> GGDPHMMFGKKKNNGGSSTARYSAGNKYNTLSNNYALSAQQLLNASKIDDIDSMMGFERYVPPQYNGRFDAKDIDQIPGRVGWLTNMHATLVSQETLSSGSNGGGNSNDGERVTTNQGISGVDFYFLDEEGGSFKSTVVYDPYFFIACNDESRVNDVEELVKKYLESCLKSLQIIRKEDLTMDNHLLGLQKTLIKLSFVNSNQLFEARKLLRPILQDNANNNVQRNIYNVAANGSEKVDAKHLIEDIREYDVPYHVRVSIDKDIRVGKWYKVTQQGFIEDTRKIAFADPVVMAFDIETTKPPLKFRDSAVDQIMMISYMIDGEGFLITNREIISEDIEDFEYTPKPEYPGFFTIFNENDEVALLQRFFEHIRDVRPTVISTFNGDFFDWPFIHNRSKIHGLDMFDEIGFAPDAEGEYKSSYCSHMDCFRWVKRDSYLPQGSQGLKAVTQSKLGYNPIELDPELMTPYAFEKPQHLSEYSVSDAVATYYLYMKYVHPFIFSLCTIIPLNPDETLRKGTGTLCEMLLMVQAYQHNILLPNKHTDPIERFYDGHLLESETYVGGHVESLEAGVFRSDLKNEFKIDPSAIDELLQELPEALKFSVEVENKSSVDKVTNFEEIKNQITQKLLELKENNIRNELPLIYHVDVASMYPNIMTTNRLQPDSIKAERDCASCDFNRPGKTCARKLKWAWRGEFFPSKMDEYNMIKRALQNETFPNKNKFSKKKVLTFDELSYADQVIHIKKRLTEYSRKVYHRVKVSEIVEREAIVCQRENPFYVDTVKSFRDRRYEFKGLAKTWKGNLSKIDPSDKHARDEAKKMIVLYDSLQLAHKVILNSFYGYVMRKGSRWYSMEMAGITCLTGATIIQMARALVERVGRPLELDTDGIWCILPKSFPETYFFTLENGKKLYLSYPCSMLNYRVHQKFTNHQYQELKDPLNYIYETHSENTIFFEVDGPYKAMILPSSKEEGKGIKKRYAVFNEDGSLAELKGFELKRRGELQLIKNFQSDIFKVFLEGDTLEGCYSAVASVCNRWLDVLDSHGLMLEDEDLVSLICENRSMSKTLKEYEGQKSTSITTARRLGDFLGEDMVKDKGLQCKYIISSKPFNAPVTERAIPVAIFSADIPIKRSFLRRWTLDPSLEDLDIRTIIDWGYYRERLGSAIQKIITIPAALQGVSNPVPRVEHPDWLKRKIAT

At the eukaryotic replication fork, the family B replicative DNA polymerases epsilon (Pol ε) and delta (Pol δ) synthesize the leading and lagging strand, respectively. The exonuclease domains of family B polymerases have several highly-conserved motifs (named Exo-motifs), which include the catalytic residues (D290, E292, D383 and D477 in yeast Pol ε). The catalytic residues serve as ligands for two metal ions, and substituting both D290 and E292 with alanine abolishes the proofreading function of the polymerase, which in turn increases the in vitro mutation rate by ~100-fold. At present, many structures of family B DNA polymerases with proofreading capacity have been determined, and their overall structures are well conserved, consisting of a thumb, palm, fingers and the exonuclease domain.

Here we report the crystal structure of the catalytic core of S. cerevisiae Pol ε with a P301R substitution, orthologous to P286R in human Pol ε. To investigate the structural and functional impact of the P301R mutation on S. cerevisiae Pol ε, the catalytic core of the Pol2 subunit of Pol ε (Pol2CORE) with the P301R substitution was purified. There were no rearrangements of the N-terminal, exonuclease, finger, palm, thumb or P-domains, nor were there any alterations in the interactions with DNA and the incoming nucleotide in the ternary complex of Pol2CORE-P301R. The P301R substitution is located in a loop, called the Exo-loop, but does not affect the overall conformation of the Exo-loop. In the Pol2CORE-P301R structure, the R301 points toward the catalytic site, forming an ion pair with E292. The R301-E292 ion pair interaction is buttressed by a water molecule that is stabilized by the backbone amide group of T293. In contrast to the wild-type, the P301R structure harbors only a Ca2+ ion in the A-site, coordinated by water molecules and three catalytic residues D290, E292 and D477. Interestingly, we observe a steric clash between the terminal residue of the ssDNA and R301, suggesting that R301 will interfere with the binding of ssDNA to the exonuclease site. Taken together, the structural and molecular dynamic simulation data show that the mechanism of exonuclease inactivation in Pol2CORE-P301R involves a steric obstruction of ssDNA binding in the exonuclease site, in addition to the loss of catalytic activity. To summarize, our structural and molecular dynamics simulation studies revealed that the cancer-associated P301R substitution prevents proper positioning of ssDNA in the exonuclease active site of Pol ε.> MDLEMMLDEDYKEGICLINFSQIALSTALVNFPDKEKINLSMVRHLILNSIKFNVKKAKTLGYTKIVLCIDNAKSGYWRRDFAYYYKKNRGKAREESTWDWEGYFESSHKVIDELKAYMPYIVMDIDKYEADDHIAVLVKKFSLEGHKILIISSDGDFTQLHKYPNVKQWSPMHKKWVK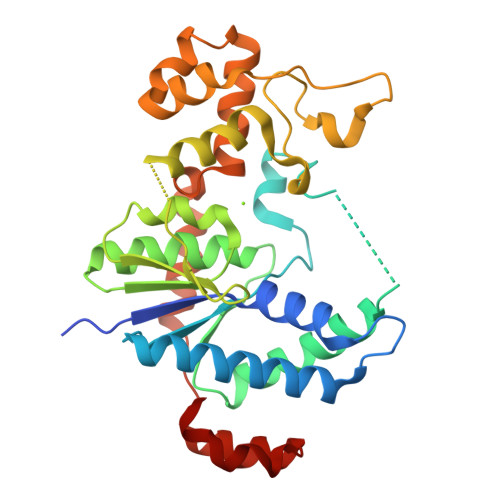IKSGSAEIDCMTKILKGDKKDNVASVKVRSDFWFTRVEGERTPSMKTSIVEAIANDREQAKVLLTESEYNRYKENLVLIDFDYIPDNIASNIVNYYNSYKLPPRGKIYSYFVKAGLSKLTNSINEF>[2x]SNAMKQAIGFIDSGVGGLTVVREVLKQLPHEQVYYLGDTARCPYGPRDKEE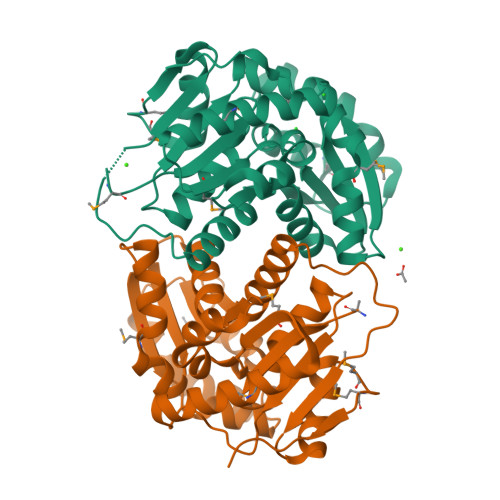VAKFTWEMTNFLVDRGIKMLVIACNTATAAALYDIREKLDIPVIGVIQPGSRAALKATRNNKIGVLGTLGTVESMAYPTALKGLNRRVEVDSLACPKFVSVVESGEYKSAIAKKVVAESLLPLKSTKIDTVILGCTHYPLLKPIIENFMGDGVAVINSGEETASEVSALLDYHNLLDATDEEIEHRFFTTGSTQIFKDIAKDWLNMPDMTVEHIKLGK(1S,4r)-4-[(1P)-5-chloro-1-(1-methyl-1H-pyrazol-4-yl)-1H-indazol-6-yl]-1-(oxetan-3-yl)piperidin-1-ium | C19 H23 Cl N5 O | 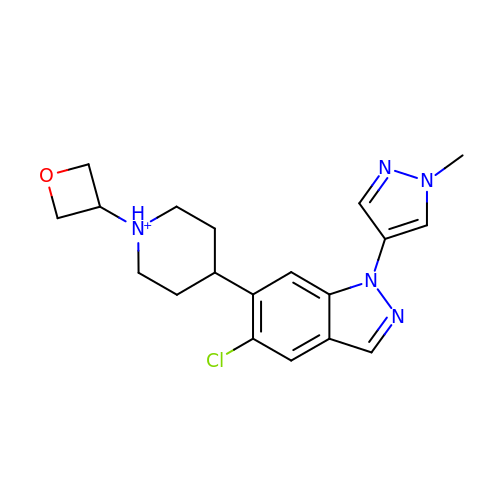QNTMOHJVKJNXDF-UHFFFAOYSA-O> ALRGTVTDFSGFDGRADAE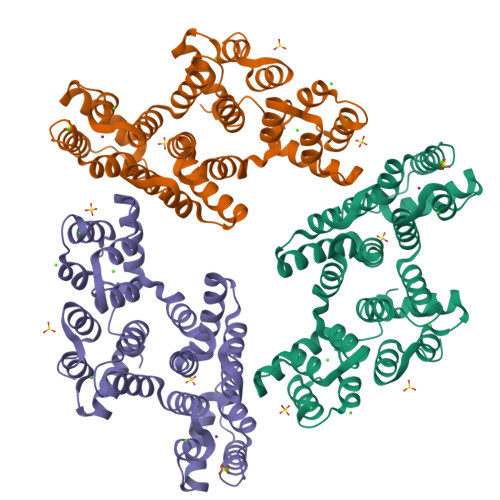VLRKAMKGLGTDEDSILNLLTARSNAQRQQIAEEFKTLFGRDLVNDMKSELTGKFEKLIVALMKPSRLYDAYELKHALKGAGTDEKVLTEIIASRTPEELRAIKQAYEEEYGSNLEDDVVGDTSGYYQRMLVVLLQANRDPDTAIDDAQVELDAQALFQAGELKWGTDEEKFITILGTRSVSHLRRVFDKYMTISGFQIEETIDRETSGNLENLLLAVVKSIRSIPAYLAETLYYAMKGAGTDDHTLIRVIVSRSEIDLFNIRKEFRKNFATSLYSMIKGDTSGDYKKALLLLCGGEDD> MELKHSISDYTEAEFLQLVTTICNADTSSEEELVKLVTHFEEMTEHPSGSDLIYYPKEGDDDSPSGIVNTVKQWRAANGKSGFKQG;> MESKRNKPGKATGKGKPVGDKWLDDAGKDSGA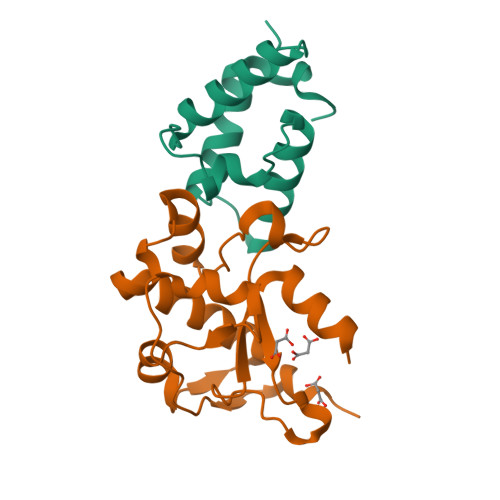PIPDRIADKLRDKEFKSFDDFAKAVWEEVSKDPELSKNLNPSNKSSVSKGYSPFTPKNQQVGGRKVYELHHDKPISQGGEVYDMDNIRVTTPKRHIDIHRGK[4-(5-chloranyl-[1,3]oxazolo[4,5-b]pyridin-2-yl)piperazin-1-yl]-[2-(4-cyclopentylpyridin-3-yl)-1,3-benzoxazol-6-yl]methanone | C28 H25 Cl N6 O3 | 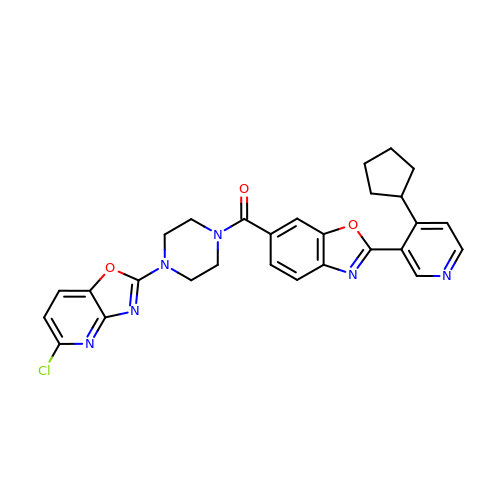RKCIAPWMPDOONC-UHFFFAOYSA-N>MSKRRKHSWPQPLKGAESRLWYGGDYNPDQWPEEVWDDDIRLMKKAGVNLVSVGIFSWAKIEPEEGKYDFDWLDRAIDKLGKAGIAVDLASATASPPMWLTQAHPEVLWKDERGDTVWPGAREHWRPTSPVFREYALNLCRRMAEHYKGNPYVVAWHVSNEYGCHNRFDYSDDAMRAFQKWCKKRYKTIDAVNEAWGTAFWAQHMNDFSEIIPPRYIGDGNFMNPGKLLDYKRFSSDALKELYIAERDVLESITPGLPLTTNFMVSAGGSMLDYDDWGAEVDFVSNDHYFTPGEAHFDEVAYAASLMDGISRKEPWFQMEHSTSAVNWRPINYRAEPGSVVRDSLAQVAMGADAICYFQWRQSKAGAEKWHSSMVPHAGEDSQIFRDVCELGADLGRLSDEGLMGTKTVKSKVAVVFDYESQWATEYTANPTQQVDHWTEPLDWFRALADNGITADVVPVRSDWDSYEIAVLPCVYLLSEETSRRVREFVANGGKLFVTYYTGLSDENDHIWLGGYPGSIRDVVGVRVEEFAPMGNDMPGALDHLDLDNGTVAHDFADVITSTADTSTVLASYKAERWTGMNE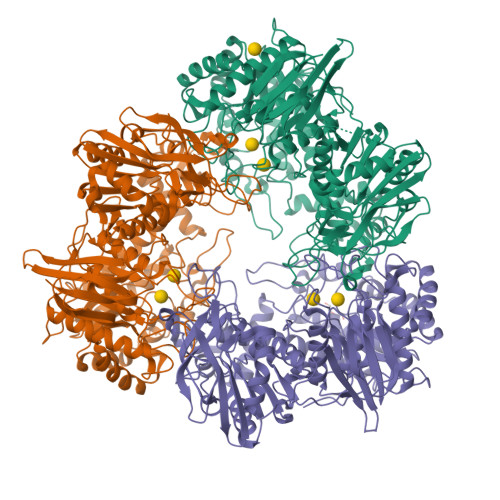VPAIVANGYGDGRTVYVGCRLGRQGLAKSLPAMLGSMGLSDLAGDGRVLRVERADAAAASHFEFVFNRTHEPVTVDVEGEAIAASLAHVDDGRATIDPTGVVVLRR[3x]> GSHMAVSQTSQTVASHVPFADLCSTLERIQKSKGRAEKIRHFREF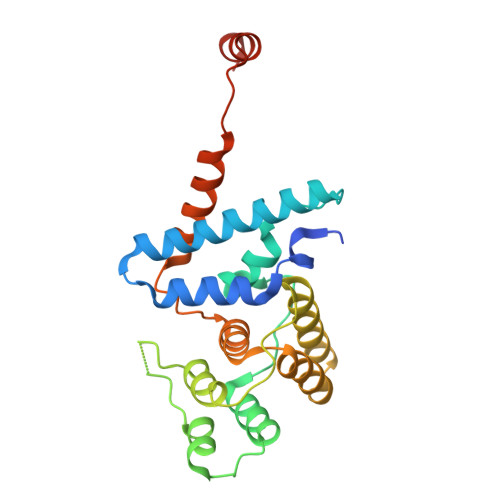LDSWRKFHDALHKNHKDVTDSFYPAMRLILPQLERERMAYGIKETMLAKLYIELLNLPRDGKDALKLLNYRTPTGTHGDAGDFAMIAYFVLKPRCLQKGSLTIQQVNDLLDSIASNNSAKRKDLIKKSLLQLITQSSALEQKWLIRMIIKDLKLGVSQQTIFSVFHNDAAELHNVTTDLEKVCRQLHDPSVGLSDISI> MAAVLESLLREEVSVAAVVRWIARSTQGSEDNAGEAAALSSLRALRKEFVPFLLNFLREQSSRVLPQGPPTPAKTPGASAALPGRPGGPPRGSRGARSQLFPPTEAQSTAAEAPLARRGGRRRGPGPARERGGRGLEEGVSGESLPGAGGRRLRGSGSPSRPSLTLSDPPNLSNLEEFPPVGSVPPGPTGTKPSRRINPTPVSEERSLSKPKTCFTSPPISCVPSSQPSALDTSPWGLGLPPGCRSLQEEREMLRKERSKQLQQSPTPTCPTPELGSPLPSRTGSLTDEPADPARVSSRQRLELVALVYSSCIAENLVPNLFLELFFVFQLLTARRMVTAKDSDPELSPAVLDSLESPLFQSIHDCVFFAVQVLECHFQVLSNLDKGTLKLLAENERLLCFSPALQGRLRAAYEGSVAKVFLVMPPSTQAVSFQPETDNRANFSSDRAFHTFKKQRDVFYEVLREW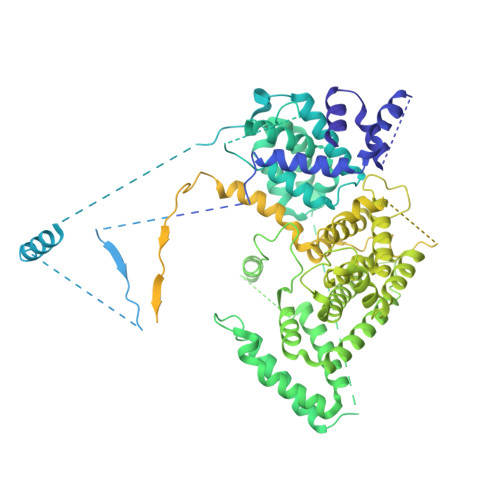EDHHEEPGWDFEKGLGSRIRAMMGQLSAACSHSHFVRLFQKQLLQMCQSPGGAGGTVLGEAPDVLSMLGADKLGRLWRLQERLMAPQSSGGPCPPPTFPGCQGFFRDFILSASSFQFNQHLMDSLSLKIQELNGLALPQHEPNDEDGESDVDWQGERKQFAVVLLSLRLLAKFLGFVAFLPYRGPEPPPTGELQDSILALRSQVPPVLDVRTLLQRGLQARRAVLTVPWLVEFLSFADHVVPLLEYYRDIFTLLLRLHRSLVLSQESEGKMCFLNKLLLLAVLGWLFQIPTVPEDLFFLEEGPSYAFEVDTVAPEHGLDNAPVVDQQLLYTCCPYIGELRKLLASWVSGSSGRSGGFMRKITPTTTTSLGAQPSQTSQGLQAQLAQAFFHNQPPSLRRTVEFVAERIGSNCVKHIKATLVADLVRQAESLLQEQLVTQGEEGGDPAQLLEILCSQLCPHGAQALALGREFCQRKSPGAVRALLPEETPAAVLSSAENIAVGLATEKACAWLSANITALIRREVKAAVSRTLRAQGPEPAARGERRGCSRACEHHAPLPSHLISEIKDVLSLAVGPRDPDEGVSPEHLEQLLGQLGQTLRCRQFLCPPAEQHLAKCSVELASLLVADQIPILGPPAQYRLERGQARRLLHMLLSLWKEDFQGPVPLQLLLSPRNVGLLADTRPREWDLLLFLLRELVEKGLMGRMEIEACLGSLHQAQWPGDFAEELATLSNLFLAEPHLPEPQLRACELVQPNRGTVLAQSLEACGTKLENLYFQ>[2x]KKQTQRNVFRCNVIGVKNCGKSGVLQALLG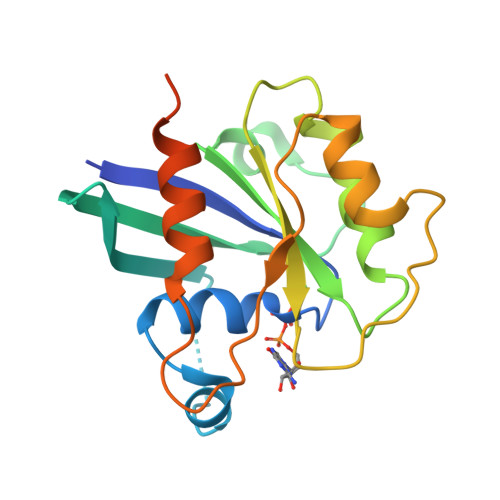RNLMRQKKIREDHKSYYAINTVYVYGQEKYLLLHDISESEFLTEAEIICDVVCLVYDVSNPKSFEYCARIFKQHFMDSRIPCLIVAAKSDLHEVKQEYSISPTDFCRKHKMPPPQAFTCNTADAPSKDIFVKLTTMAMYPHVTQADLKSSTFLEHHHHHH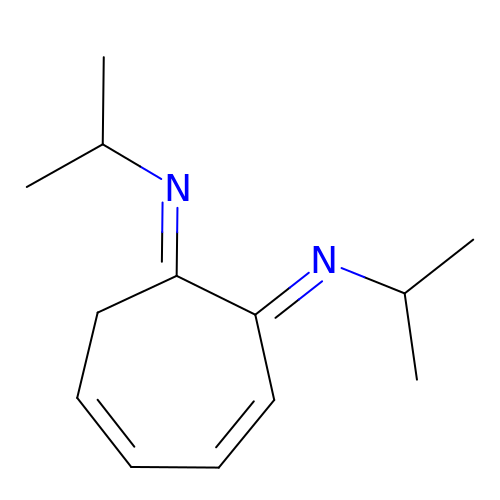(1E,2E)-N,N'-di(propan-2-yl)cyclohepta-3,5-diene-1,2-diimine | C13 H20 N2 | WTKTZDHSCKRTLA-QUMQEAAQSA-N>[2x]GGGRNFTVLRKLNLVPIKKSVSSPKVCKPSPVKERVDHVFYQKFKSMALQELGTNYLSISYVPSLSKFLSKNLRSMKNCIVFFDKVEHIHQYAGIDRAVSETLSLVDINVVIIEMNDYLMKEGIQSSKSKECIESMGQASYSGQLDFEASEKPSNHTSDLMMMVMRKINNDESIDHIVYFKFEQLDKLSTSTIIEPSKLTEFINVLSVLEKSNNIAFKVLIYSNNVSISSLLSTSLKKKLNTKYTVFEMPILT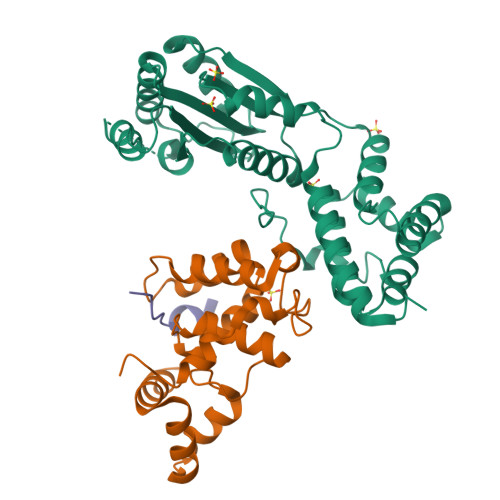CAQEQEYLKKMIKFTFDSGSKLLQSYNSLVTCQLNNKESNLAIFFEFLKVFPHPFTYLFNAYTEIIVQSRTFDELLDKIRNRLTIKNYPHSAYNFKKNQRLPLKLTRKVHDR;>[2x]GASNSYAIPENELLDEDTMNFISSLKNDLSNISNSLPFEYPHEIAEAIRSDFSNEDIYDNIDPDTISFPPKIATTDLFLPLFFHFGSTRQFMDKLHEVISGDYEPSQAEKLVQDLCDETGIRKNFSTSILTCLSGDLMVFPRYFLNMFKDNVNPPPNVPGIWTHDDDESLKSNDQEQIRKLVKKHGTGRMEMRKRFFEKDLL;>[2x]FTVLRKLNLVPIK>[4x]GADLADRFAELERRYDARLGVYVPATGTTAAIEYRADERFAFCSTFK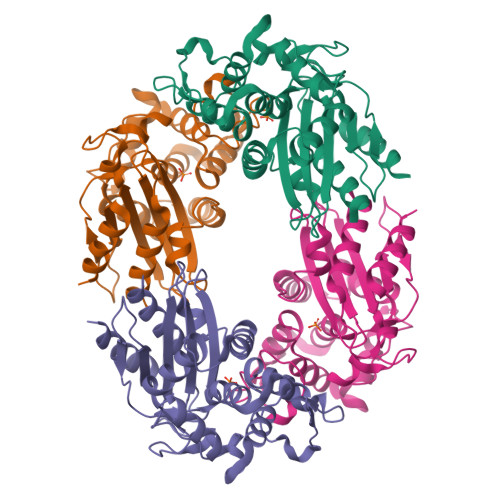APLVAAVLHQNPLTHLDKLITYTSDDIRSISPVAQQHVQTGMTIGQLCDAAIRYSDGTAANLLLADLGGPGGGTAAFTGYLRSLGDTVSRLDAEEPELNRDPPGDERDTTTPHAIALVLQQLVLGNALPPDKRALLTDWMARNTTGAKRIRAGFPADWKVIDKTGTGDYGRANDIAVVWSPTGVPYVVAVMSDRAGGGYDAEPREALLAEAATCVAGVLA>SSLKEKFAEYEAFGPRILELWQAARNAFEAGDLARVANLLAELKELFKKDLNLANAMAAE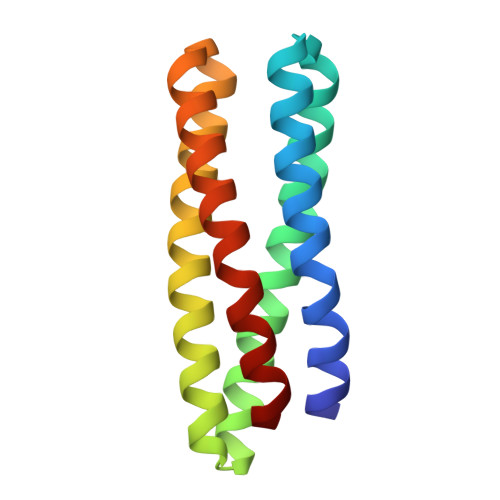AAEAGNKEAVALLAEQLERLKKIQAMFAAAVNAFRAGDREAFGALLEAIINEGKALLPLVEAIKEAI[6x]>[8x]MGDRGPEFVATTVELPLQQKADAAQTVTGPLPFGNSLLKEFVLDPAYRNLNHGSFGTIPSAIQQKLRSYQTAAEARPCPFLRYQTPV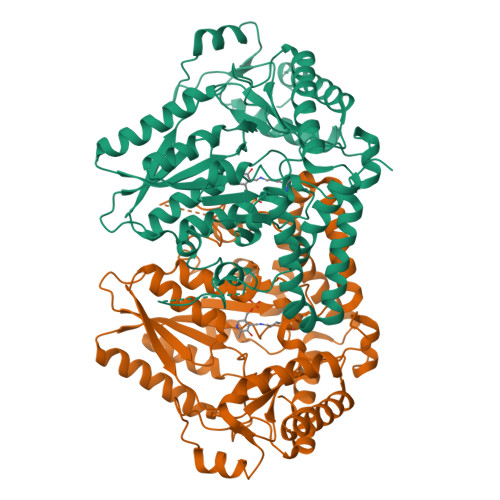LLDESRAAVANLLKVPVETVVFVANATMGVNTVLRNIVWSADGKDEILYFDTIFGACGKTIDYVIEDKRGIVSSRCIPLIYPAEDDDVVAAFRDAIKKSREEGKRPRLAVIDVVSSMPGVRFPFEDIVKICKEEEIISCVDGAQGIGMVDLKITETDPDFLISNCHKWLFTPRGCAVFYVPVRNQHLIRSTLPTSHGFVPQVGNRFNPLVPAGNKSAFVSNFEFVGTVDNSPFFCVKDAIKWREEVLGGEERIMEYMTKLAREGGQKVAEILGTRVLENSTGTLIRCAMVNIALPFVVGEDPKAPVKLTEKEEKDVEGLYEIPHEEANMAFKWMYNVLQDEFNTFVPMTFHRRRFWARLSAQVYLEMSDFEWAGKTLKELCERVAKGEYKESALEVDLQGDHGLSAWSHPQFEK>[2x]GAMVSQPIKLLVGLADPGPEYAKTRHNAGAWVVEELAR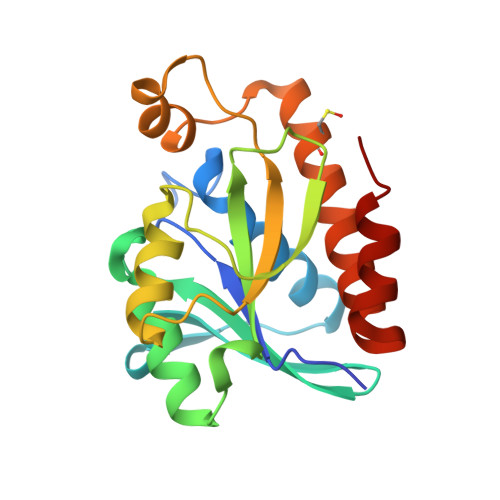IHNVTLKNEPKFFGLTGRLLINSQELRVLIPTTFMNLSGKAIAALANFYQIKPEEIMVAHDELDLPPGVAKFKQGGGHGGHNGLKDTISKLGNNKEFYRLRLGIGHPGHKDKVAGYVLGKAPAKEQECLDAAVDESVRCLEILMKDGLTKAQNRLHTFKAE>[4x]SEKEKVEELAQRIREQLPDTELAREAQELADEARKSDDSEALKVVYLALRIVQQLPDTELAREALELAKEAVKSTDSEALKVVYLALRIVQQLPDTELARLALELAKKAVEMTAQEVLEIARAALKAAQAFPNTELAELMLRLAEVAARVMKELERNDEEIKKSDELDDESLLEDIVELLKEIIKLWKILVEVSDVMLKLIS;>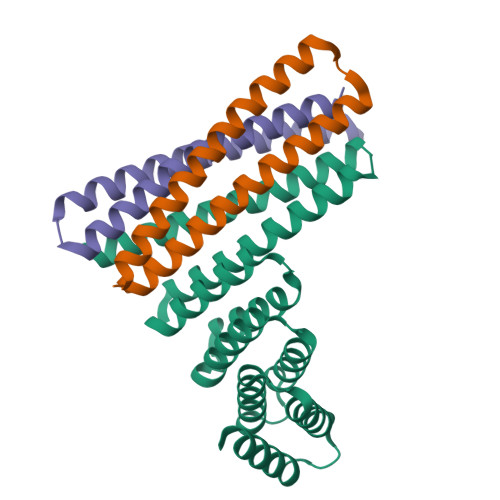[4x]GPVDEIDKEVKKLEEEAKKSQEEVERLKQEVEKASKAGLDHEGDSRIFKKIHDVVTKQIKVILRLIAVYAELVAIIG;>[4x]GSKQKEAIKVYLELLEVHSRVLKALIEQIKLFIELIKRPDEDLADKVRKSSEELKKIIKEVEKILRKVDDILYKVKS> MSGLRPPARQLITPLSEEWRSRVEAARNANPATELAKTLEGQPLVRRDFEEKLLPATAWLNDNVIIGAIFYIADYVNTKKGAPNQEPKCTAFTSFFWPRLLSHGPGGCGRLLRRANVRKANFLDIDTILIP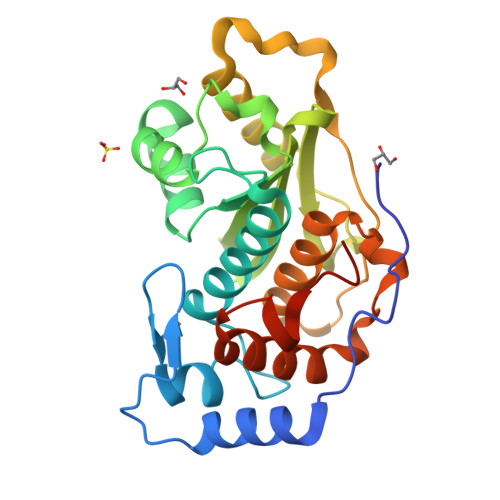ICESSHWTLAVIRPGRRTVSHLDSMAAGRGSERVKAKLLELVKFVLEDQFVEAEWQAVDFQAPRQTNGWDCGVFTITNAICLALGVDPAQAYTEAQLPLQRQRIAAVLLNGGFKGDFTLDDLHHHHHHHHHH> MGETITVSTPIKQIFPDDAFAETIKDNLKKKSVTDAVTQNELNSIDQIIANNSDIKSVQGIQYLPNVTKLFLNGNKLTDIKPLTNLKNLGWLFLDENKIKDLSSLKDLKKLKSLSLEHNGISDINGLVHLPQLESLYLGNNKITDITVLSRLTKLDTLSLEDNQISDIVPLAGLTKLQNLYLSKNHISDLRALAGLKNLDVLELFSQECLNKPINHQSNLVVPNTVKNTDGSLVTPEIISDDGDYEKPNVKWHLPEFTNEVSFIFYQPVTIGKAKARFHGRVTQPLKEVYTVSYDVDGTVIKTKVEAGTRITAPKPPTKQGYVFKGWYTEKNGGHEWNFNTDYMSGNDFTLYAVFKAETTEKTVNLTRYVKYIRGNAGIYKLPREDNSLKQGTLASHRCKALTVDREARNGGKLWYRLKNIGWTKAENLSLDRYDKMEYDKGVTAYARVRNASGNSVWTKPYNTAGAKHVNKLSVYQGKNMRILREAKTPITTWYQFSIGGKVIGWVDTRALNTFYKQSMEKPTRLTRYVSANKAGESYYKVPVADNPVKRGTLAKYKNQKLIVDCQATIEGQLWYRIRTSSTFIGWTKAANLRAQKLE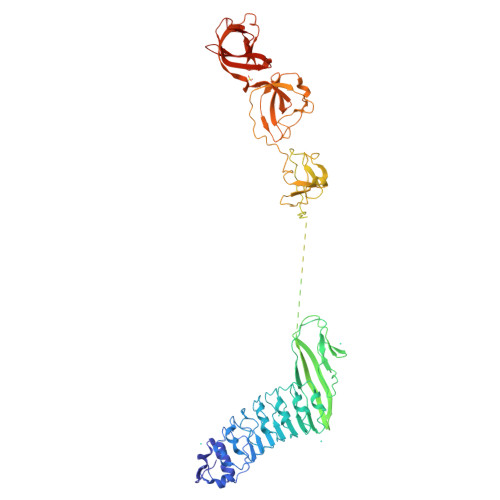HHHHHH> MGKMFFVDLSRCTACRGCQIACKQWKNLPAEETRNTGSHQNPPDLSYVTL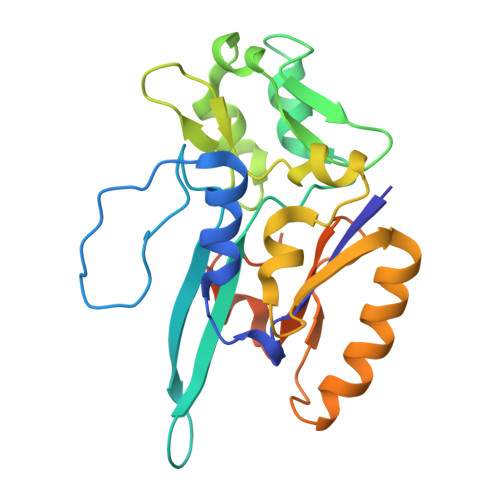KTVRFTEKSRKGPGIDWLFFPEQCRHCVEPPCKGQADVDLEGAVVKDETTGAVLFTELTAKVDGESVRSACPYDIPRIDPVTKRLSKCDMCNDRVQNGLLPACVKTCPTGTMNFGDEQEMLALAEKRLAEVKKTYPGAVLGDPNDVRVVYLFTRDPKDFYEHAVADLAPSMMTRQQLFARLFRPRA>[3x]GPRSACAEPLRRQDVRKTVDKLVEHHIDTQQISPYILSRSLEDYVRSFDSHKAYLTQDEVFSHAFSEEATHPLFKQYQEDNFSSFKELDTCIQQSISRAREWRSSWLTDSIRVIQDAMSHTIEKKPSAWASSIEEVKQRQYDLLLSYASIYLEDAAKNRYQGKEHGLVKLCIRQIENHENPYIGINDHGYRMSPEEEANSFHVRIIKSIAHSLDAHTAYFSQEEALSMRAQLEKGMCGIGVVLKEDIDGVVVKEVLAGGPADKTGSLRVGDIIYRVNGKNIENTPFPGVLDSLRGSPGSSVTLDIHRQNNDHVIQLRREKILLDSRRVDVSYEPYGNGIIGKITLHSFYEGENQVSSEQDLRKAIRELQEKNLLGLVLDIRENTGGFLSQAIKVSGLFLTNGVVVVSRYADGSVKRYRTISPQKFYDGPLAVLVSKSSAAAAEIVAQTLQD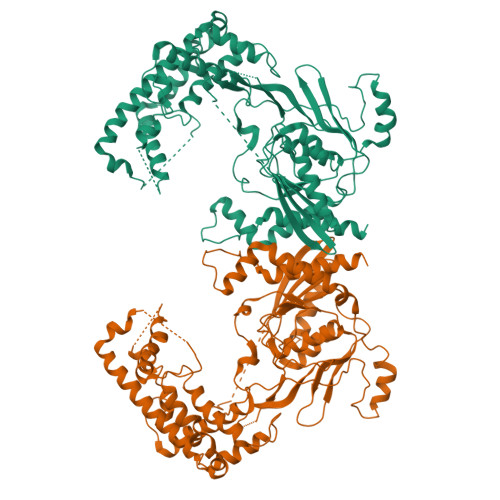YGVALIVGDQQTYGKGTIQHQTITGSNSQEDFFKVTVGRYYSPSGKSTQLEGVKSDIVIPSRYAEDKLGERFLEYALPADQYDNVINDNLGDLDINIRPWFQKYYSPHLQKPELVWREMLPQLAHNSQERLEKNKNFEIFVQHLKKTNKQDRSFGSNDLQMEESVNIVKDMILLKSISQTPAQ4-{6-amino-5-[4-(methylsulfonyl)phenyl]pyridin-3-yl}phenol 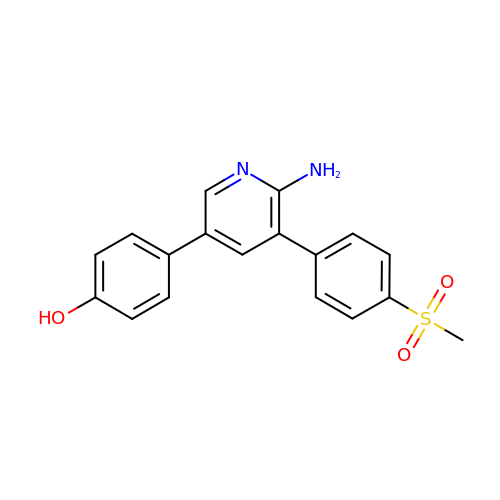| C18 H16 N2 O3 S | XFEKSSMJINNJSX-UHFFFAOYSA-N> MKHHHHHHHGAAGTSLYKKAGLVPRGSMNPQLYLCASVFITRGDVKSVSEIYQGLQSDAERLQYLKLLCVMWPELDAPTNISFVLKDIELNGMDESSVLVSLIQEDSSLTAISEMDVNTISKRVNALASYVEETLIGFNIHIRETHMLEDFIRARTLVVNSLSKDALCSLELLANSTSKSLVSWLDGILKPLDHLNRRLDTKLSIFQFENLSAQDAVSEMWKLPVKEVSVVRSMMKYEVEPYLKFQGSYTPFYEVIFNPDNFPLDSINNFQIYKYLSSQPTPLDTKFNETKWNILYSNGKNLASIPLPNLVFELESLIKSFGDDSQIFSGISLNEWLVNLKFMNAMDIKDLKSLKKLQNEDSVVQTSYFSIITQNMFQGHIDIKTVQNVVEFIESSTLFDKLTNELQTSILLESLLKLGKFDILEQFVSTSGVKIQDKVIIQHFWRFFNIASNGSLSDPDMKNANRTLNLLSNKETHSNLYDILTIVDRLSHYSLSFKRGMPFKPAHISEFKANPMEIVEKLLDLNPKLRKNIEVTFDILKELYTALQVTPSDKDFTKEYSKLLSEHINNLLANGDFKFAFDQAINLIERPDAAEHWVTIFQVGKYIDPNWLDAEIPTEIIYLQLGIVSKLLHICPEKEYEVI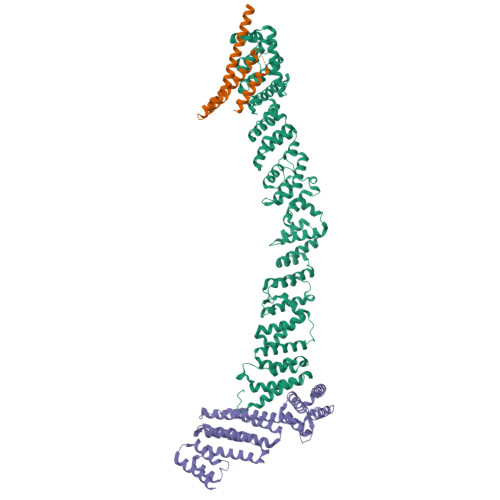TSQWSGLELELSTRNLISDKYSLENTQRSNDNFMSDVSTNVGNFLSGKFQWNIGGA;> MGSMTTDLDTLSDQLRKNYYRDLSLFQDDEDPFYHYLISTKLATNLNTVRKLAIKDNLDDPSSDAIDRYQKNFSRLEESVSSISFSKASKLQQKYDAYQESQKKRRYSVDFDA;> MGSENIYTTLKFESMMQQRVIQIRSIPEEEYHELVSVQGDGDGPIQVSVFVQSAAKVFTEFEQGCDTIGRSKVESIYLYKFNLLQTAFFAMVSEKVNDWTQLYKDVRYLYTENPKLLQLMELNSRRLDLNLNLIKKTIYKLVNDQLQELKDNERTPDWDITISSLLPYLKKTALPTLYKLEDNTILVALIRYIVHDLVIDNILHWRVISEKSSENLSEFIMLLLSGLEIPRLNLIETYRHSREKLGILSKILTAHLKDILEMFYEGEFFLFETDEIVQWIILLFADTPTRRDCIDEIRRVREEATD>GAMELGSLCQGDSMQGQLKLGCIPTIAPFLLCDLVQEINQRFPQLNLLLREDTTTNLLTALRHGELDVLILALPVEIDGMESRVVGQDPFKMVISRHQAGAIKVPIKYDDLPDESVFLLEKGHCLTEHAVSACKLTDKEKINPFSATSLHTLVQMVANGLGTTFIPQMAIDHGLLDNQNLVVIEPPGQQAYRDIGLVWRPSSSRSKTFNQLAEVVS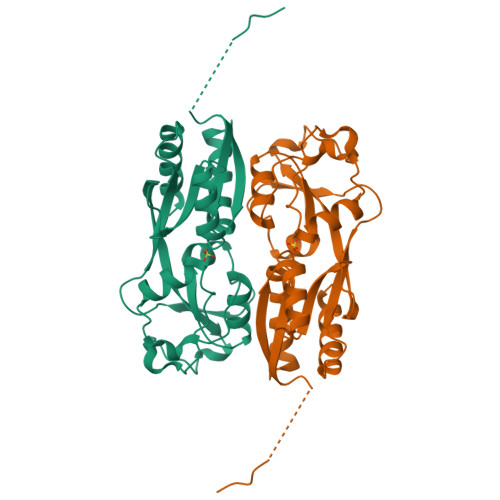ELL[2x]> TFVSCPGAPQPRYQMNVANGFRVAPVLGGLTMPRGITLDTRGNLLVVERGRGLTGHTLDANGCVTSSKVVIQDTQINHGIDVHPSGRRIIASSGDIAWSWDYDPATMTATNRRTLVTGMNNFYHFTRTVHISRKYPNLFALNVGSDGNIDVPTRQQNSGRAQIRVFDYDQLPQNGVPFVSQYGRVLGYGLRNDVGITEDRAGNIHSIENSLDNAYRMVNGQRRDIHTNNPAEKVYNLGDPSNPRAIFGGYPDCYTVWEPSDFTDSPKQPGDWFTQDNSGQYTDAWCNANAVKPTLLLPPHTAPLDMKFGLGNDTNLYVALHGSWNRQPPQGYKVVVVPGQYSASGEWSPTAPLAQSRTAWSDLLTNRNENQCSGFGNANCFRPVGL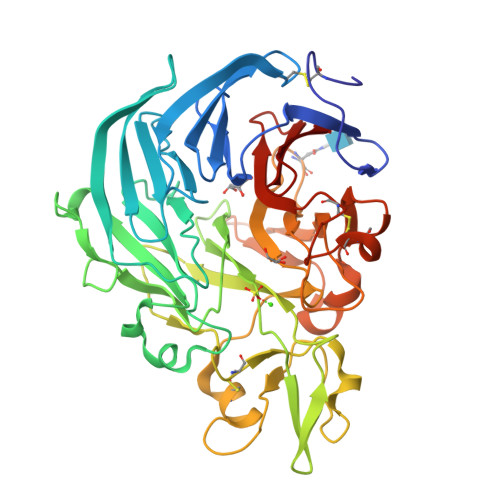VWSADGQNLYVSSDTSGEVFIIKR> QRATKM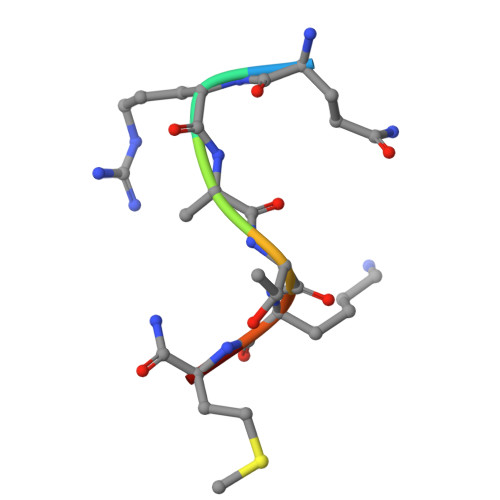X>MHHHHHHSTPSIVIASAARTAVGSFNGAFANTPAHELGATVISAVLERAGVAAGEVNEVILGQVLPAGEGQNPARQAAMKAGVPQEATAWGMNQLCGSGLRAVALGMQQIATGDASIIVAGGMESMSMAPHCAHLRGGVKMGDFKMIDTMIKDGLTDAFYGYHMGTTAENVAKQWQLSRDEQDAFAVASYNKAEAAQKDGRFKDEIVPFIVKGRKGDITVDADEEIRGATLDKMAKLRPAFDKEGTVTAGNASTLNDGAAAALLMSEAEASRRGIQPLGRIVSWATVGVDPKVMGTGPIPASRKALER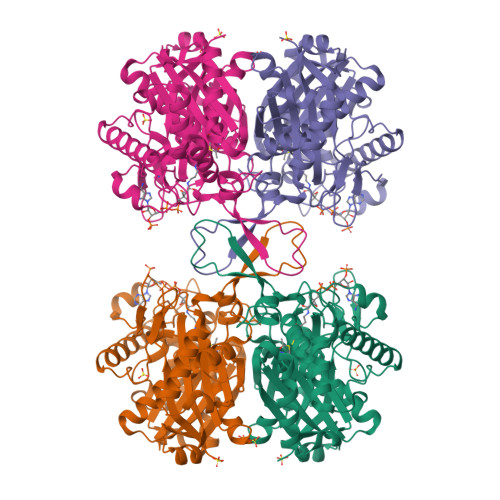AGWKIGDLDLVEANEAFAAQACAVNKDLGWDPSIVNVNGGAIAIGHPIGASGARILNTLLFEMKRRGARKGLATLCIGGGMGVAMCIESL[4x]>XGEIAKALREIAKALREIAWAHR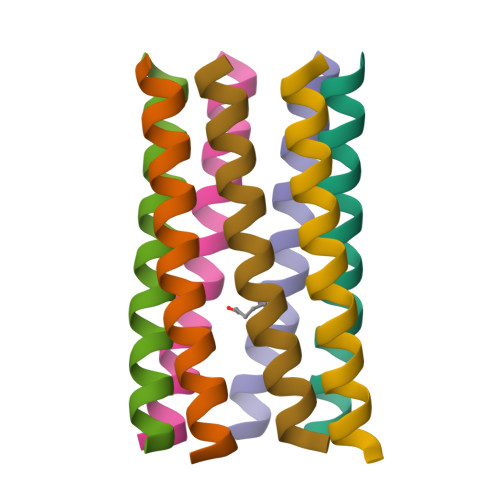EIAKALRG[7x]> AQVINTFDGVADYLQTYHKLPNDYITKSEAQALGWVASKGNLADVAPGKSIGGDIFSNREGKLPGKSGRTWRE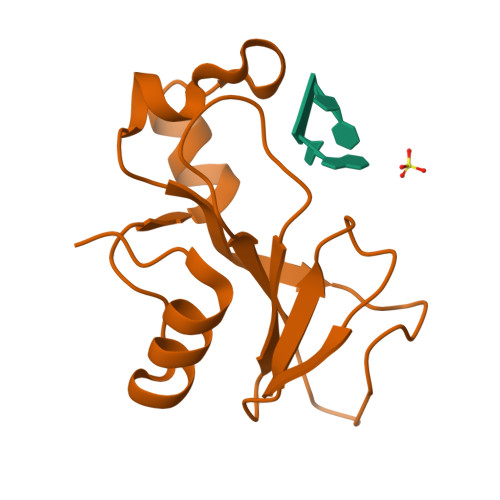ADINYTSGFRNSDRILYSSDWLIYKTTDHYQTFTKIR(3~{R})-1-phenylpyrrolidine-3-carboxylic acid | C11 H13 N O2 | 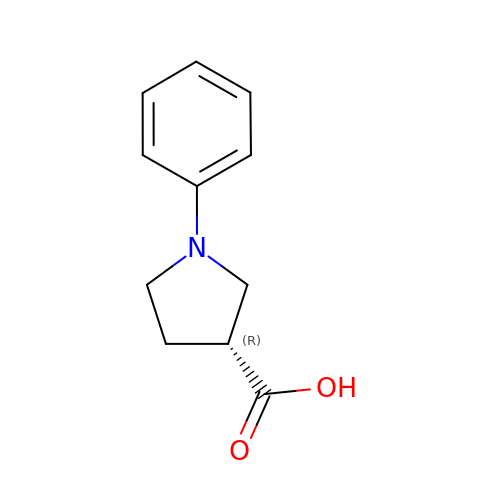IOFLKIRLUFZCHR-SECBINFHSA-N>MIKLCREVWIEVNLDAVKKNLRAIRRHIP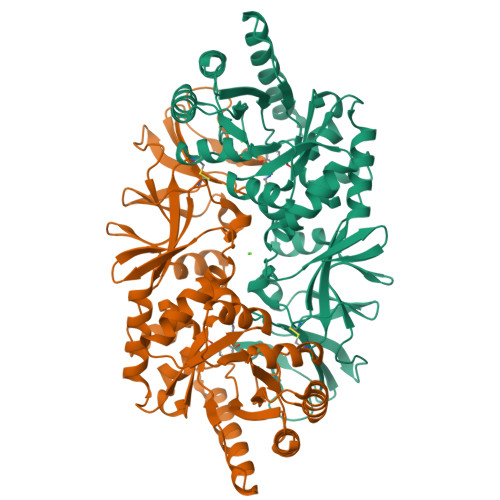HKSKIMAVVKANGYGHGSIEVARHALEHGASELAVASVEEGIVLRKAGITAPILVLGFTSLSCVKKSAAWNITLSAFQVDWMKEANEILEKEASANRLAIHINVDTGMGRLGVRTKEELLEVVKALKASKFLRWTGIFTHFSTADEPDTTLTKLQHEKFISFLSFLKKQGIELPTVHMCNTAAAIAFPEFSADMIRLGIGLYGLYPSAYIKQLNLVKLEPALSLKARIAYVKTMRTEPRTVSYGATYIAEPNEVIATLPIGYADGYSRALSNRGFVLHRGKRVPVAGRVTMDMIMVSLGENGEGKQGDEVVIYGKQKGAEISVDEVAEMLNTINYEVVSTLSRRIPRFYIRDGEIFKVSTPVLYV[2x]> MAARLLAPPGPDSFKPFTPESLANIERRIAESKLKKPPKADGSHREDDEDSKPKPNSDLEAGKSLPFIYGDIPQGLVAVPLEDFDPYYLTQKTFVVLNRGKTLFRFSATPALYILSPFNLIRRIAIKILIHSVFSMIIMCTILTNCVFMTFSNPPDWSKNVEYTFTGIYTFESLVKIIARGFCIDGFTFLRDPWNWLDFSVIMMAYITEFVNLGNVSALRTFRVLRALKTISVIPGLKTIVGALIQSVKKLSDVMILTVFCLSVFALIGLQLFMGNLRNKCVVWPINFNESYLENGTKGFDWEEYINNKTNFYTVPGMLEPLLCGNSSDAGQCPEGYQCMKAGRNPNYGYTSFDTFSWAFLALFRLMTQDYWENLYQLTLRAAGKTYMIFFVLVIFVGSFYLVNLILAVVAMAYEEQNQATLEEAEQKEAEFKAMLEQLKKQQEEAQAAAMATSAGTVSEDAIEEEGEEGGGSPRSSSEISKLSSKSAKERRNRRKKRKQKELSEGEEKGDPEKVFKSESEDGMRRKAFRLPDNRIGRKFSIMNQSLLSIPGSPFLSRHNSKSSIFSFRGPGRFRDPGSENEFADDEHSTVEESEGRRDSLFIPIRARERRSSYSGYSGYSQGSRSSRIFPSLRRSVKRNSTVDCNGVVSLIGGPGSHIGGRLLPEATTEVEIKKKGPGSLLVSMDQLASYGRKDRINSIMSVVTNTLVEELEESQRKCPPCWYKFANTFLIWECHPYWIKLKEIVNLIVMDPFVDLAITICIVLNTLFMAMEHHPMTPQFEHVLAVGNLVFTGIFTAEMFLKLIAMDPYYYFQEGWNIFDGFIVSLSLMELSLADVEGLSVLRSFRLLRVFKLAKSWPTLNMLIKIIGNSVGALGNLTLVLAIIVFIFAVVGMQLFGKSYKECVCKINQDCELPRWHMHDFFHSFLIVFRVLCGEWIETMWDCMEVAGQAMCLIVFMMVMVIGNLVVLNLFLALLLSSFSADNLAATDDDGEMNNLQISVIRIKKGVAWTKLKVHAFMQAHFKQREADEVKPLDELYEKKANCIANHTGADIHRNGDFQKNGNGTTSGIGSSVEKYIIDEDHMSFINNPNLTVRVPIAVGESDFENLNTEDVSSESDPEGSKDKLDDTSSSEGSTIDIKPEVEEVPVEQPEEYLDPDACFTEGCVQRFKCCQVNIEEGLGKSWWILRKTCFLIVEHNWFETFIIFMILLSSGALAFEDIYIEQRKTIRTILEYADKVFTYIFILEMLLKWTAYGFVKFFTNAWCWLDFLIVAVSLVSLIANALGYSELGAIKSLRTLRALRPLRALSRFEGMRVVVNALVGAIPSIMNVLLVCLIFWLIFSIMGVNLFAGKYHYCFNETSEIRFEIEDVNN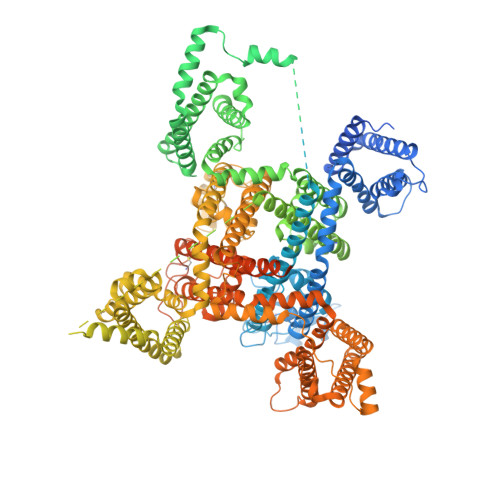KTECEKLMEGNNTEIRWKNVKINFDNVGAGYLALLQVATFKGWMDIMYAAVDSRKPDEQPKYEDNIYMYIYFVIFIIFGSFFTLNLFIGVIIDNFNQQKKKFGGQDIFMTEEQKKYYNAMKKLGSKKPQKPIPRPLNKIQGIVFDFVTQQAFDIVIMMLICLNMVTMMVETDTQSKQMENILYWINLVFVIFFTCECVLKMFALRHYYFTIGWNIFDFVVVILSIVGMFLADIIEKYFVSPTLFRVIRLARIGRILRLIKGAKGIRTLLFALMMSLPALFNIGLLLFLVMFIFSIFGMSNFAYVKHEAGIDDMFNFETFGNSMICLFQITTSAGWDGLLLPILNRPPDCSLDKEHPGSGFKGDCGNPSVGIFFFVSYIIISFLIVVNMYIAIILENFSVATEESADPLSEDDFETFYEIWEKFDPDATQFIEYCKLADFADALEHPLRVPKPNTIELIAMDLPMVSGDRIHCLDILFAFTKRVLGDSGELDILRQQMEERFVASNPSKVSYEPITTTLRRKQEEVSAVVLQRAYRGHLARRGFICKKTTSNKLENGGTHREKKESTPSTASLPSYDSVTKPEKEKQQRAEEGRRERAKRQKEVRESKC>MTIMAPEAVGESLDPRDPLLRLSNFFDDGSVELLHERDRSGVLAAAGTVNGVRTIAFCTDGTVMGGAMGVEGCTHIVNAYDTAIEDQSPIV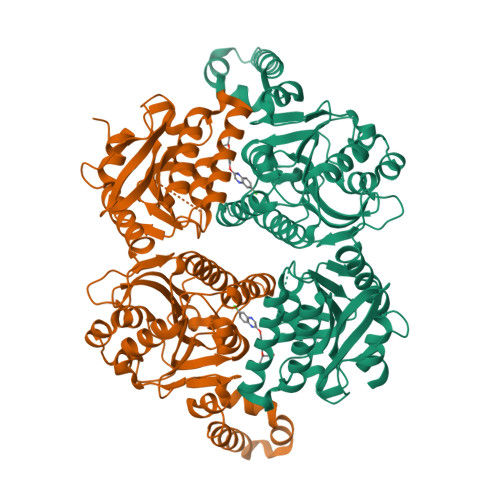GIWHSGGARLAEGVRALHAVGQVFEAMIRASGYIPQISVVVGFAAGGAAYGPALTDVVVMAPESRVFVTGPDVVRSVTGEDVDMASLGGPETHHKKSGVCHIVADDELDAYDRGRRLVGLFCQQGHFDRSKAEAGDTDIHALLPESSRRAYDVRPIVTAILDADTPFDEFQANWAPSMVVGLGRLSGRTVGVLANNPLRLGGCLNSESAEKAARFVRLCDAFGIPLVVVVDVPGYLPGVDQEWGGVVRRGAKLLHAFGECTVPRVTLVTRKTYGGAYIAMNSRSLNATKVFAWPDAEVAVMGAKAAVGILHKKKLAAAPEHEREALHDQLAAEHERIAGGVDSALDIGVVDEKIDPAHTRSKLTEALAQAPARRGRHKNIPL[4x]(4aR,6R,8aS)-8a-(2,4-difluorophenyl)-6-(1H-pyrazol-4-yl)-4,4a,5,6,8,8a-hexahydropyrano[3,4-d][1,3]thiazin-2-amine | C16 H16 F2 N4 O S | 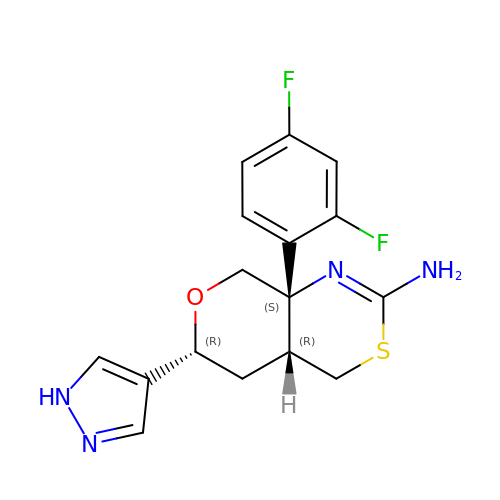KLYAOLDBWRAAEM-JJMVLAAESA-N>[2x]YVSDVYCEVC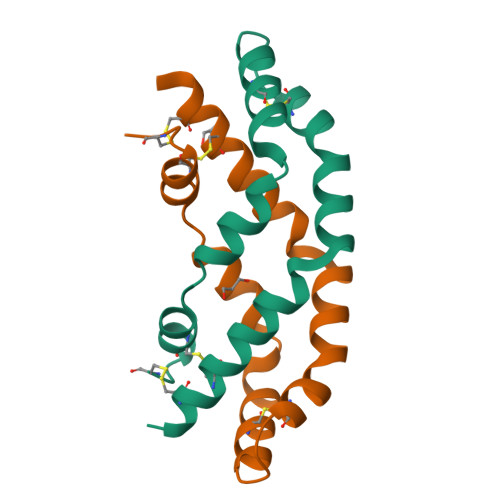EFLVKEVTKLIDNNKTEKEILDAFDKMCSKLPKSLSEECQEVVDTYGSSILSILLEEVSPELVCSMLHLCSRHHHHHH> GPHMLERYSKVDLLALRYSPLSQTPPGIELEGRLRR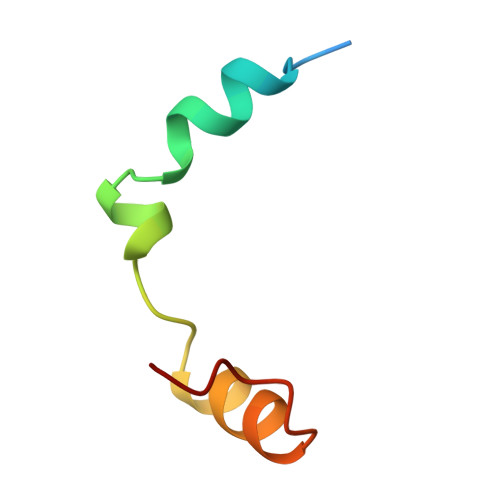MNIWRTGS> TYKATHEFMSGTPGKELPQEVKDLLPADQTDLKDGSQATPTQPSKTEVKTAEGTWSFKSYDKTSETINGADAHFVGTWEFTPAPTYKATHEFVSGTPGKELPQEVKDLLPADQTDLKDGSQATPTQPSKTEVKTTEGTWSFKSYDKTSETINGADAHFVGTWEFTPA

Here, we show that repeat number variation in predicted bacterial surface proteins is more widespread and we characterize a third rod-like repetitive region in the Streptococcus gordonii protein (Sgo_0707) formed by tandem array of Streptococcal High Identity Repeats in Tandem (SHIRT) domains. The structure of single and tandem SHIRT domains from the streptococcal surface protein Sgo_0707 were determined. We call SasG, Rib, and Sgo_0707 “Periscope Proteins” due to their having variable-length stalk-like regions that define the distance that the N-terminal functional domain projects from the bacterial surface. Taken together, these data are consistent with multiple tandemly arrayed SHIRT domains from Sgo_0707 behaving as an elongated, rod-like particle.

The structure reveals two complete domains with a very short (Pro-Ala-Pro) linker; the structure of Sgo_R3-4 is ordered throughout (residues 623 through 789). Each domain adopts the SHIRT fold, and the interdomain interface is limited; this was confirmed by comparing the Tm of Sgo_R3 (75.7 °C) and Sgo_R3-4 (76.6 °C). The similarity of unfolding curves for single and double SHIRT constructs suggests that the two domains in the tandem construct unfold independently. Notably, there is a significant twist between domains when viewed along the long axis of the molecule. Small angle X-ray scattering (SAXS) analysis substantiates the anisotropic head-to-tail domain arrangement in solution. Molecular dynamics (MD) simulations of the Sgo_R3-4 construct show that individual domains are particularly stable (rmsd <1.5 Å for Cα atoms) over the length of the trajectory (0.8 μs); their individual length is conserved during the simulation and the length of Sgo_R3-4 fluctuates only moderately around 97 Å. Consistent with the models, the Dmax that was determined using SAXS scales with the number of domains; Sgo_R3-4 exhibits a Dmax of 107 Å and Sgo_R2-8 has a Dmax of 371 Å. Like Rib, there is no evidence for significant interdomain interfaces in tandem arrays of SHIRT domains.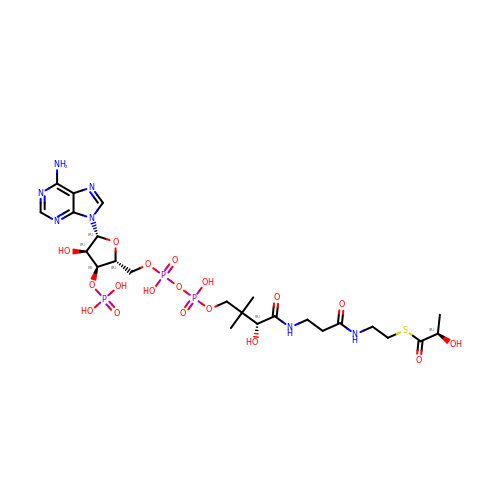S-{(3S,5R,9R)-1-[(2R,3S,4R,5R)-5-(6-amino-9H-purin-9-yl)-4-hydroxy-3-(phosphonooxy)oxolan-2-yl]-3,5,9-trihydroxy-8,8-dimethyl-3,5,10,14-tetraoxo-2,4,6-trioxa-11,15-diaza-3lambda~5~,5lambda~5~-diphosphaheptadecan-17-yl} (2R)-2-hydroxypropanethioate | C24 H40 N7 O18 P3 S | VIWKEBOLLIEAIL-AGCMQPJKSA-N> GGTGGGGCCGGCCCCACC

Nine new crystal structures of CG-rich DNA 18-mers with the sequence 5′-GGTGGGGGC-XZ-GCCCCACC-3′, which are related to the bacterial repetitive extragenic palindromes, are reported. All 18-mers crystallized as isomorphic tetragonal crystals with one strand of a right-handed antiparallel duplex in the asymmetric unit. All reported structures co-crystallized with the Sr2+ cation located between nucleotides 6 and 7 and (by symmetry) 12 and 13.

All four Chom-18-mers with two central nucleotides (residues 9 and 10) able to form Watson–Crick pairs were crystallized. Base pairs A–T and T–A are classified as Watson–Crick pairs, while the C–G pair adopts a specific orientation characterized by a large value of one of the base parameters, shear (2.97 Å), and is not classified. NtC classes provided valuable help with building the initial models of six of the nine 18-mers, i.e. Chom-18-AT, Chom-18-CG, Chom-18-GC, Chom-18-GT, Chom-18-TC and Chom-18-AG. Although the number of unassigned steps remained the same in the Chom-18-TC structure, the average confal score and the average RSCC improved. The r.m.s.d.s between the NtC-restrained and nonrestrained models were 0.45 and 0.57 Å for the Chom-18-TC and Chom-18-CG structures, respectively. Only Chom-18-CG, Chom-18-GC and Chom-18-AC have all dinucleotides assigned (classified as NtC classes AA##); unassigned dinucleotides (NtC class NANT) are mostly localized near the central base pair.> MSEVVKKFMYLNRKAPYGTIYAWEALEVVLIGAAFDQDVCVLFLDDGVYQLTRGQDTKGIGMKNFSPTYRTLGDYEVRRIYVDRDSLEARGLTQDDLVEIAFEDMETEEEFDNIVEVIDSARV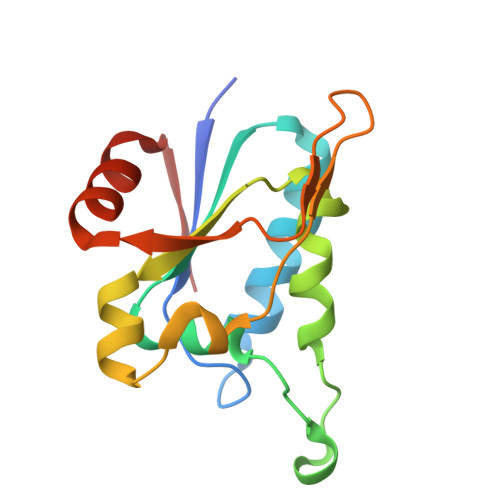SELMNESDAVFSF> MGSDKIHHHHHHMSVNLKGRSLLTLLDFSPEEIRYLLDISKQVKMENRSKLRTERFKGMTLAMIFEKRSTRTRLAFETAFAEEGGHPIFLSPNDIHLGAKESLEDTARVLGRMVDAIMFRGY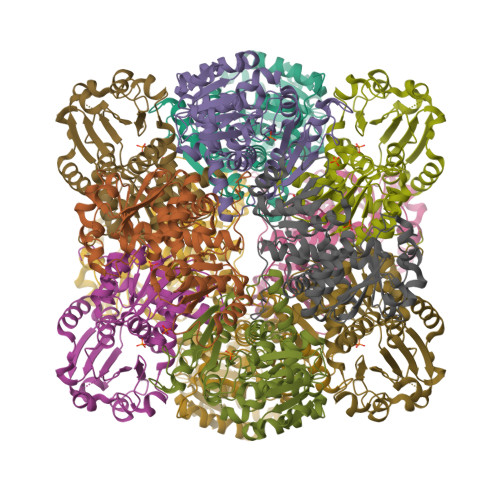KQETVEKLAEYSGVPVYNGLTDEFHPTQALADLMTIEENFGRLKGVKVVFMGDTRNNVATSLMIACAKMGMNFVACGPEELKPRSDVFKRCQEIVKETDGSVSFTSNLEEALAGADVVYTDVWASMGEEDKEKERMALLKPYQVNERVMEMTGKSETIFMHCLPAVKGQEVTYEVIEGKQSRVWDEAENRKHTIKAVMIATLL>[8x]MGSSHHHHHHGLVPRGSHMSTEITHHQAMINGYRMHYVTAGSGYPLVLLHGWPQSWYEWRNVIPALAEQFTVIAPDLRGLGDSEKPMTGFDKRTMATDVRELVSHLGYDKVGVIGHDWGGSVAFYFAYDNRDLVERLFILDMIPGLIKAGDSFPIPVALMINHIFFHGGNPDWATALISKDVNLYLRRFLT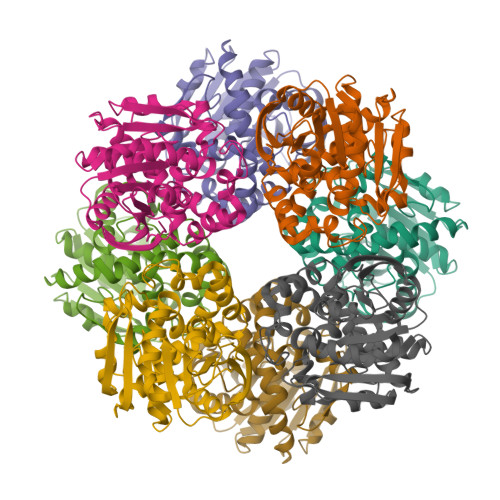TLDYNYSPNVFSEEDIAEYVRVNSLPGSIRSGCQWYATGLREDTENLAKATDKLTIPVIAWGGSHFLGDIRPAWQEVAENVEGGAVENCGHFVPEEKPQFVIDTALKFFAPLR>MGHHHHHHQQLASFLSGTWQSGRGRSRLIHHAISGEALWEVTSEGLDMAAARQFAIEKGAPALRAMTFIERAAMLKAVAKHLLSEKERFYALSAQTGATRADSWVDIEGGIGTLFTYASLGSRELPDDTLWPEDELIPLSKEGGFAARHLLTSKSGVAVHINAFNFPCWGMLEKLAPTWLGGMPAIIKPATATAQLTQAMVKSIVDSGLVPEGAISLICGSAGDLLDHLDSQDVVTFTGSAATGQMLRVQPNIVAKSIPFTMEADSLNCCVLGEDVTPDQPEFALFIREVVREMTTKAGQKCTAIRRIIVPQALVNAVSDALVARLQKVVVGDPAQEGVKMGALVNAEQRADVQEKVNILLAAGCEIRLGGQADLSAAGAFFPPTLLYCPQPDETPAVHATEAFGPVATLMPAQNQRHALQLACAGGGSLAGTLVTADPQIARQFIADAARTHGRIQILNEESAKESTGHGSPLPQLVHGGPGRAGGGEELGGLRAVKHYMQRTAVQGSPTMLAAISKQWVRGAKVEEDRIHPFRKYFEEL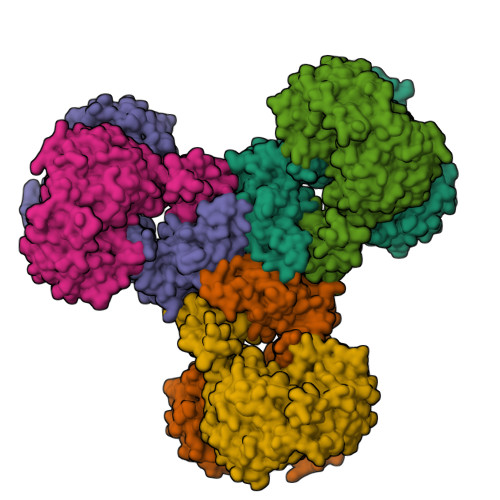QPGDSLLTPRRTMTEADIVNFACLSGDHFYAHMDKIAAAESIFGERVVHGYFVLSAAAGLFVDAGVGPVIANYGLESLRFIEPVKPGDTIQVRLTCKRKTLKKQRSAEEKPTGVVEWAVEVFNQHQTPVALYSILTLVARQHGDFVD[6x]5-HYDROXYAMINO-3-METHYL-PYRROLIDINE-2-CARBOXYLIC ACID | C6 H12 N2 O3 | 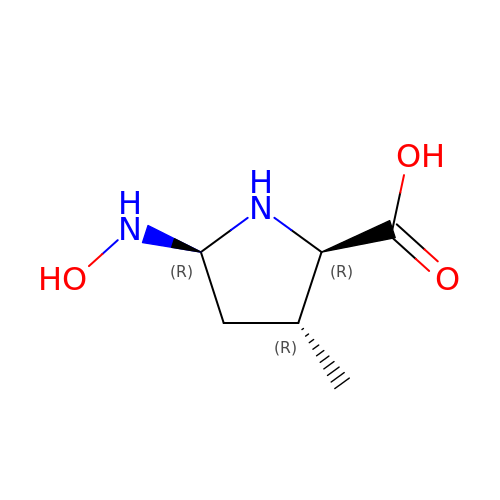PEFGUPQPFCDBPY-UOWFLXDJSA-N>GSHMASNKYKRIFLVVMDSVGIGEAPDAEQFGDLGSDTIGHIAEHMNGLQMPNMVKLGLGNIREMKGISKVEKPLGYYTKMQEKSTGKDTMTGHWEIMGLYIDTPFQVFPEGFPKELLDELEEKTGRKIIGNKPASGTEILDELGQEQMETGSLIVYTSADSVLQIAAHEEVVPLDELYKICKIARELTLDEKYMVGRVIARPFVGEPGNFTRTPNRHDYALKPFGRTVMNELKDSDYDVIAIGKISDIYD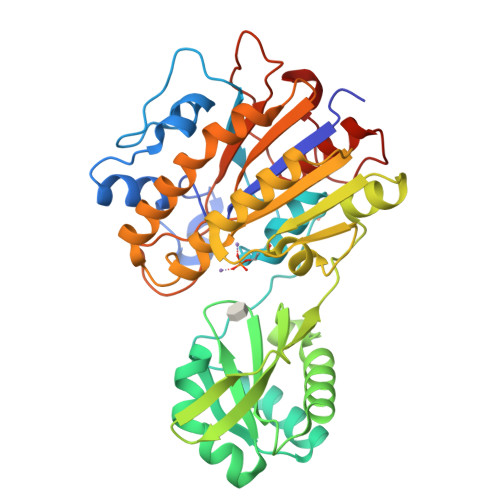GEGVTESLRTKSNMDGMDKLVDTLNMDFTGLSFLNLVDFDALFGHRRDPQGYGEALQEYDARLPEVFAKLKEDDLLLITADHGNDPIHPGTDHTREYVPLLAYSPSMKEGGQELPLRQTFADIGATVAENFGVKMPEYGTSFLNELKK[3x]>GAMGRRLGVMGGTFDPIHYGHLVAASEVADLFDLDEVVFVPSGQPWQKGRQVSAAEHRYLMTVIATASNPRFSVSRVDIDRGGPTYTKDTLADLHALHPDSELYFTTGADALASIMSWQGWEELFELARFVGVSRPGYELRNEHITSLLGQLAKDALTL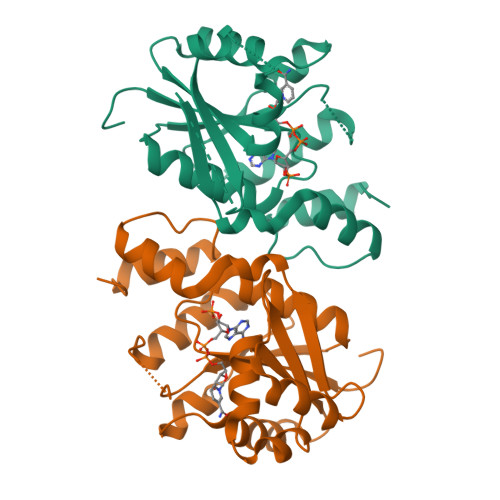VEIPALAISSTDCRQRAEQSRPLWYLMPDGVVQYVSKRRLYT[4x]> MKTQVAIIGAGPSGLLLGQLLHKAGIDNVILERQTPDEVLGRIRAGVLEQGMVDLLREAGVDRRMARDGLVHEGVEIAFAGQRRRIDLKRLSGGKTVTVYGQTEVTRDLMEAREASGATTVYQAAEVRLHDLQGERPYVTFERDGERLRLDCDYIAGCDGFHGISRQSIPAERLKVFERVYPFGWLGLLADTPPVSHELIYANHPRGFALCSQRSATRSRYYVQVPLTEKVEDWSDERFWTELKARLPAE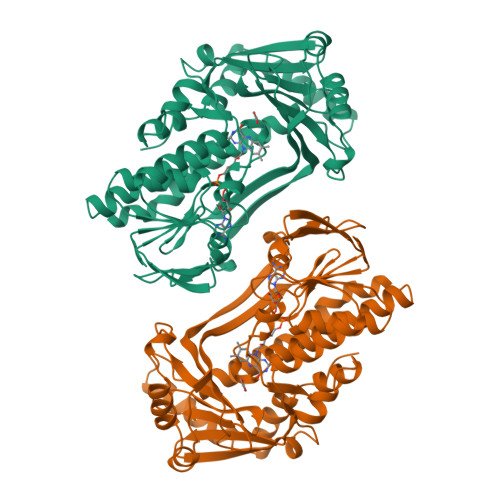VAEKLVTGPSLEKSIAPLRSFVVEPMQHGRLFLAGDAAHIVPPTGAKGLNLAASDVSTLYRLLLKAYREGRGELLERYSAICLRRIWKAERFSWWMTSVLHRFPDTDAFSQRIQQTELEYYLGSEAGLATIAENYVGLPYEE> GSHMSHEQFRAALQLVVDPGDPRSYLDNFIKIGEGSTGIVCIATVRSSGKLVAVKKMDLRKQQRRELLFNEVVIMRDYQHENVVEMYNSYLVGDELWVVMEFLEGGALTDIVTHTRMNEEQIAAVCLAVLQALSVLHAQGVIHRDIKSDSILLTHDGRVKLSDFGFCAQVSKEVPRRKSLVGTPYWMAPELISRLPYGPEVDIWSLGIMVIEMVDGEPPYFNEPPLKAMKMIRDNLPPRLKNLHK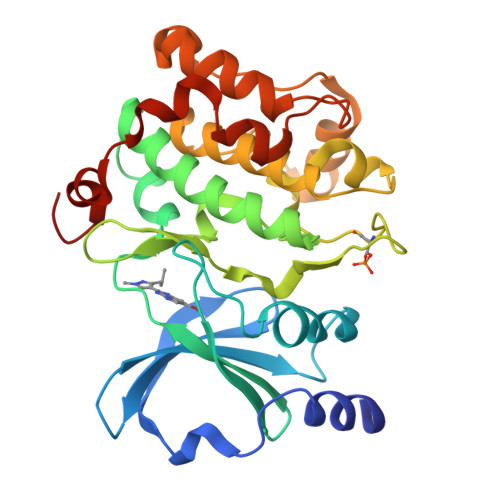VSPSLKGFLDRLLVRDPAQRATAAELLKHPFLAKAGPPASIVPLMRQNRTR>[2x]MIENSSPYTSEHFHYTVTDIKDLTKLGAIYDKTKKYWVYQGKPVMPDQFTFELLDF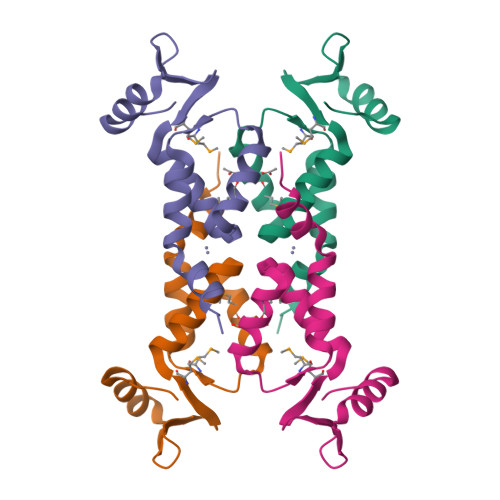LHQLTHLSFSKMKALLERSHSPYYMLNRDRTLKNITETCKACAQVNASKSLEHHHHHH> YEVKFVEAYASLFKSRLSKLKRILRENPEISNVVDIGKLNYVSGDEEVTIIGLVNSKRETNRGLIFEVEDKTGIVKVFLPKDSEDYREAFKVLPDAVVAFKGFYSKKGIFFANKFYLPDVPLYRKQKPPLEEKVYAILISDIHVGSREFCEKAFLKFLEWLNGHVESKEEEEIVSRVKYLIIAGDVVDGIGIYPGQYSDLVIPDIFDQYEALANLLANVPEHITMFIGPGNADAARPAIPQPEFYKEYAKPIYKLKNAIIISNPAVIRLHGRDFLIAHGRGIEDVVSFVPGLTHHKPGLPMVELLKMRHLAPTFGGKVPIAPDPEDLLVIEEVPDLVQMGHVHVYDAVVYRGVQLVNSATWQAQTEFQKMVNIVPTPAKVPVVDVESARVVKVLDFSGWC;> MELPKEMEEYFEMLQREIDKAYEIAKKARAQGKDPSLDVEIPQATDMAGRVESLVGPPGVAKRIRELVKEYGKEIAALKIVDEIIEGKFGDLGSREKYAEQAVRTALAILTEGIVSAPIEGIANVKIKRNTWADNSEYLALYYAGPIRSSGGTAQALSVLVGDYVRRKLGLDRFKPSEKHIERMVEEVDLYHRAVTRLQYHPSPEEVRLAMRNIPIEITGEATDDVEVSHRDVPGVETNQLRGGAILVLAEGVLQKAKKLVKYIDKMGIEGWEWLKEFVEAKEKGEPKEEGKEESLAESTLEETKVEVDMGFYYSLYQKFKEEIAPSDKYAKEVIGGRPLFSDPSKPGGFRLRYGRSRASGFATWGINPATMILVDEFLAIGTQLKTERPGKGAVVTPVTTIEGPIVKLKDGSVLRVDDYNLALKVREDVEEILYLGDAVIAFGDFVENNQTLLPANYCEEWWILEFVKALKEIYEVHLEPFTENEEESIEEASDYLEIDPEFLKEMLRDPLRVKPPVELAIHFSEVLGIPLHPYYTLYWNSVEPKDVEKLWRLLKNYAEIEWSNFRGIKFAKKIVISQEKLGDSKRTLELLGLPHTVRDGNVIVDYPWA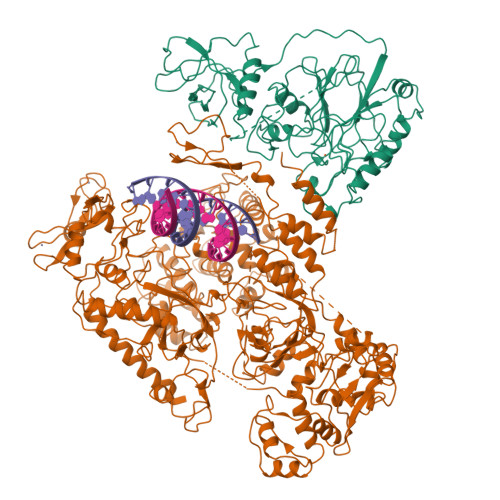AALLTPLGNLNWEFMAKPLYATIDIINENNEIKLRDRGISWIGARMGRPEKAKERKMKPPVQVLFPIGLAGGSSRDIKKAAEEGKVAEVEIAFFKCPKCGHVGPEHLCPNCGTRKELLWVCPRCNAEYPESQAEGYNYTCPKCNVKLRPYAKRKIRPSELLNRAMENVKVYGVDKLKGVMGMTSGWKMPEPLEKGLLRAKNDVYVFKDGTIRFDATDAPITHFRPREIGVSVEKLRELGYTHDFEGKPLVSEDQIVELKPQDIILSKEAGRYLLKVAKFVDDLLEKFYGLPRFYNAEKMEDLIGHLVIGLAPHTSAGIVGRIIGFVDALVGYAHPYFHAAKRRNCDGDEDAVMLLLDALLNFSRYYLPEKRGGKMDAPLVITTRLDPREVDSEVHNMDIVRYYPLEFYEATYELKSPKELVGVIERVEDRLGKPEMYYGLKFTHDTDDIALGPKMSLYKQLGDMEEKVRRQLEVAKRIRAVDEHGVAEKILNSHLIPDLRGNLRSFTRQEFRCVKCNTKFRRPPLNGKCPVCGGKIVLTVSKGAIEKYLGTAKMLVTEYNVKNYTRQRICLTERDIDSLFENVFPETQLTLIVNPNDICQRLVMARTGEVNKSGLLENLSNGSKKTEKAEKAEKPRKKSDEKPKKKRVISLEEFFSRKSK> MGSSHHHHHHSQDPMVLLHKSTHIFPTDFASVSRAFFNRYPNPYSPHVLSIDTISRNVDQEGNLRTTRLLKKSGKLPTWVKPFLRGITETWIIEVSVVNPANSTMKTYTRNLDHTGIMKVEEYTTYQFDSATSST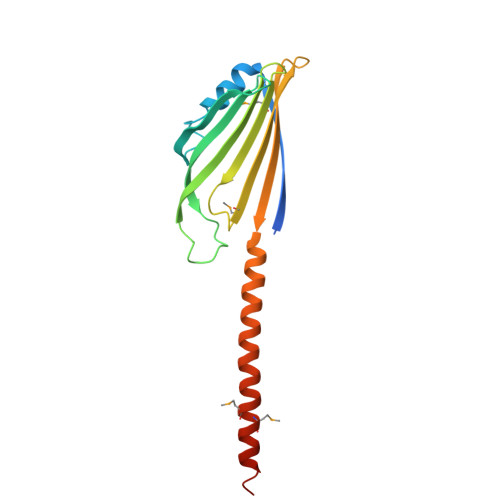IADSRVKFSSGFNMGIKSKVEDWSRTKFDENVKKSRMGMAFVIQKLEEARNPQF>[2x]MEKFLVIAGPNAIESEELLLKVGEEIKRLSEKFKEVEFVFKSSFDKANRSSIHSFRGHGLEYGVKALRKVKEEFGLKITTDIHESWQAEPVAEVADIIQIPAFLCRQTDLLLAAAKTG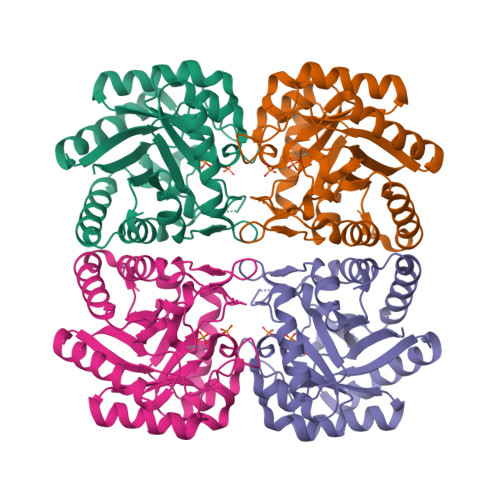RAVNVKKGQFLAPWDTKNVVEKLKFGGAKEIYLTERGTTFGYNNLVVDFRSLPIMKQWAKVIYDATHSVQLPGGLGDKSGGMREFIFPLIRAAVAVGCDGVFMETHPEPEKALSDASTQLPLSQLEGIIEAILEIREVASKYYETIPVK>[4x]MPQLHYVPYDTPVEDVMRILKESGTLVIRNFLDQNTVQKVQDEVDDYVRNWNPGPKYNHDIKNVGSKTKQPSNLSLMSKTYRCEVLNHPWMHAICERMFGPTYGDYWFNGGSILHLEPGENT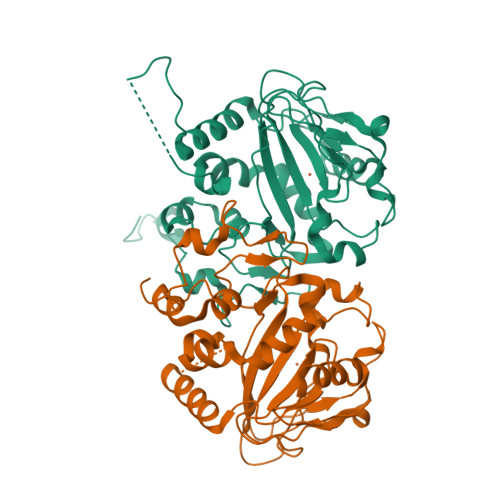QPIHQDHVFYQISKWRRPTDPDLTINFTMALTEFTVENGGTRVCPGSHLWENGHASPAEEDMVPVLMQPGDALILPGSMWHSAGANRTSEYRRGFATSFHPCHFTPIESHHHLPREMVEEMTPLVQKMLGFRTLNLHNNVKVWKAGEGNLEDATGLKSVAAKLAAALEHHHHHH> ASMTGNECPELQPPVHGKIEPSQAKYFFKDQVLVSCDTGYKVLKDNVEMDTFQIECLKDGTWSNKIPTCKIVDCRAPGELEHGLITFSTRNNLTTYKSEIKYSCQEPYYKMLNNNTGIYTCSAQGVWMNKV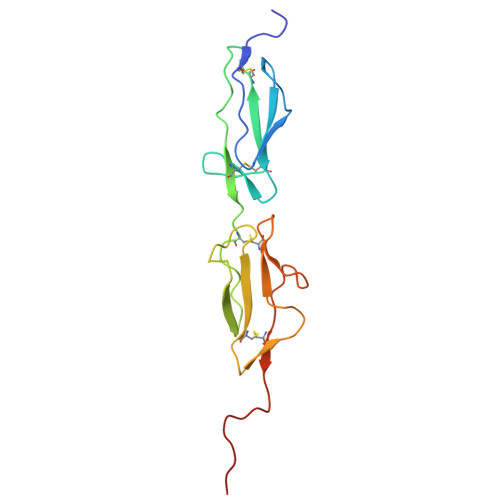LGRSLPTCLPVCGLPKFSRKLMAR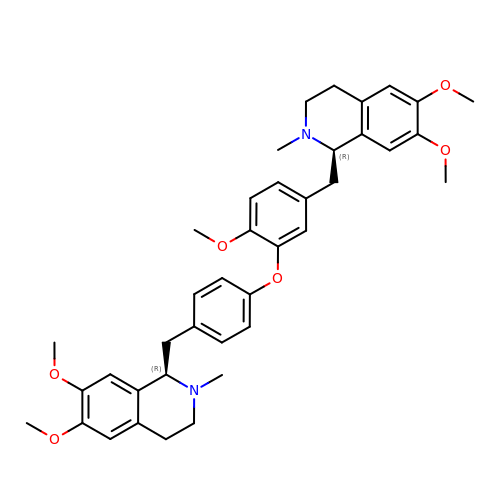(1~{R})-1-[[4-[5-[[(1~{R})-6,7-dimethoxy-2-methyl-3,4-dihydro-1~{H}-isoquinolin-1-yl]methyl]-2-methoxy-phenoxy]phenyl]methyl]-6,7-dimethoxy-2-methyl-3,4-dihydro-1~{H}-isoquinoline | C39 H46 N2 O6 | UHYCXSGUNAWVBW-CZNDPXEESA-N>HMTGERPFSCEFCEQRFTEKGPLLRHVASRHQEGRPHFCQICGKTFKAVEQLRVHVRRHKGVRKFECTECGYKFTRQAHLRRHMEIHDRVENYNPRQRKLR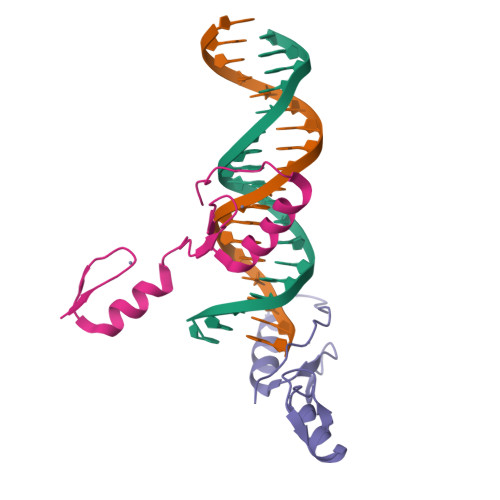NLIIED[2x]> GAMGSVSCEECGGGHSPSKLLLCDKCDRGYHLFCLR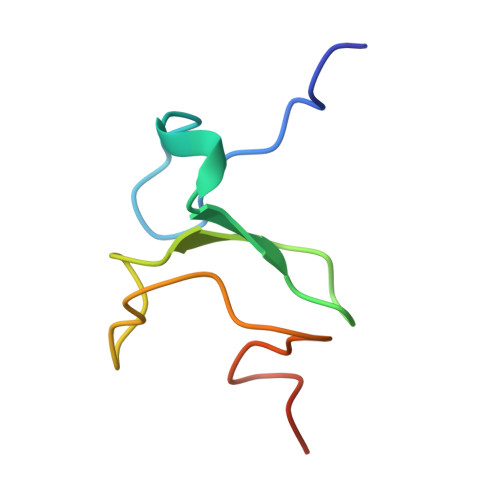PILPSVPKGSWFCPSCSNHKPK>GPLGSPIGVFW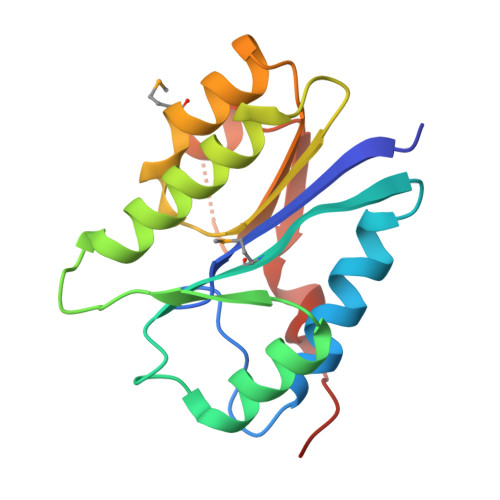DIENCSVPSGRSATAVVQRIREKFFKGHREAEFMCVCDISKENKEVIQELNNCQVTVAHINATAKNAADDKLRQSLRRFANTHTAPATVVLVSTDVNFAMELSDLRHRHGFHIILVHKNQASEALLHHANELIRFEEFISDLPHHHHHH[2x]Thus, in the deep-sea bacterium Myroides profundi D25, TMA is taken into the cells through a TMA transporter TmaT and then oxidized to TMAO, resulting in the accumulation of intracellular TMAO to millimolar levels to function as a piezolyte. TmaT is a member of the betaine-choline-carnitine transporter family, and we show that TmaT is an Na+/TMA symporter, which possessed high specificity and binding affinity toward TMA. TmaT forms a homotrimer structure in solution. Each TmaT monomer has 12 transmembrane helices, and the TMA transport channel is formed by a four-helix bundle.

To probe the transport mechanism of TmaT, we further solved two structures of TmaT-TMA complexes, TmaT-TMA LCI and TmaT-TMA LCII, in which TMA is located in different binding sites. In comparison to the electron densities of TmaT, additional electron densities at the potential TMA-binding sites were observed in the TmaT-TMA complexes, indicating the positions of TMA molecules. The TMA-binding site in TmaT-TMA LCI corresponds to the betaine-binding site I in BetP, while the TMA-binding site in the TmaT-TMA LCII corresponds to the betaine-binding site II in BetP. Analysis of the TmaT-TMA LCI structure indicated that when TMA is located at the substrate-binding site I (LCI), it is surrounded by four aromatic amino acid residues (Trp146, Trp151 and Tyr154 from TM4, and Trp326 from TM8), forming an aromatic box. In the structure of TmaT-TMA LCII, the TMA molecule is positioned at the second substrate-binding site (LCII), which is downstream of LCI within the substrate transport channel. The LCII is also composed by three aromatic residues (Trp325, Trp326, and Trp329 in TM8). Comparison of the TmaT-TMA LCI and TmaT-TMA LCII structures revealed that when TMA enters the aromatic box at the LCII site, the side chain of Trp326 flips inward and acts as a lid to control the opening and closing of the aromatic box. Upon comparing the structures of TmaT-TMA LCI and TmaT-TMA LCII, it is evident that the proximity of TM3 and TM7 resulted in the closure of the substrate channel. Analysis of the structures of TmaT-TMA LCI and TmaT-TMA LCII suggests that after the binding of TMA, the hydrogen bond formed between residues Ser95 and Asn262 may play a crucial role in the transition between these two conformations. The overall structures of TmaT, TmaT-TMA LCI, and TmaT-TMA LCII monomers are similar, with the RMSD values ranging from 0.4 to 0.7 Å.

>[3x]MFKKLLDNKNLVINPPVFITSILLIVALILTCVLFPEKVGVWFPAAQLAVTSNFGWFFVVTVNVILIFAIYLAFSKFGRIRLGGDDAEPEFTKASWFAMLFSTGMGIGIMFFSIAEPVSHFFNTPRPVDTDIEAAVQAMQFTSLHWGLHAWGIYAMVGLALAFFGFNRKLPMTFRSLFYPFWGERIHGWWGHIIDILSALATVFGLSTSLGLGVIQITAGLEYLYGWEISPMMQAGIILFVIGIATISVFSGLDKGVKILSNANMYIAASFMLLIFILGPTLFIMKGYVENTGAYLANFIDISTWNDTYLGSGWQNVWTIFYWAWWIAWSPFVGSFIARISKGRTVKEFVLGVLIVPGLITLLWMNVFGGSALHTILSGDVTMIAAVKADVSTALFVFLENFPFTKFLSIVAIILIFSFFITSSDSGSLVVDNITSGSNGESPVWQRVFWSFAQGIIAIVLLWGGGLDALQTAVIITGLPFAVILLVMCYSLQKGLKEELAKSSKKAKSKEEKSYKEIIAELLDEPQSKHHHHHHHHHH>[2x]MDLTVEPNLHSLITSTTHKWIFVGGKGGVGKTTSSCSIAIQMALSQPNKQFLLIS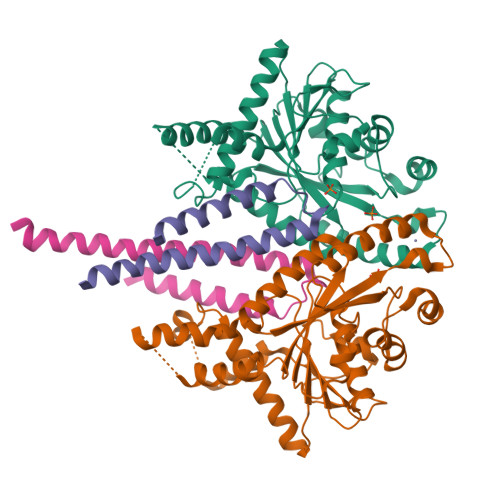TDPAHNLSDAFGEKFGKDARKVTGMNNLSCMEIDPSAALKDMNDMAVSRANNNGSDGQGDDLGSLLQGGALADLTGSIPGIDEALSFMEVMKHIKRQEQGEGETFDTVIFDTAPTGHTLRFLQLPNTLSKLLEKFGEITNKLGPMLNSFMGAGNVDISGKLNELKANVETIRQQFTDPDLTTFVCVCISEFLSLYETERLIQELISYDMDVNSIIVNQLLFAENDQEHNCKRCQARWKMQKKYLDQIDELYEDFHVVKMPLCAGEIRGLNNLTKFSQFLNKEYNPITDGKVIYELEDKELEHHHHHH;>[2x]MQYTNKYHEKWISKFAPGNELSKKYLAKVKERHELKEFNNSISAQDNYAKWTKNNRKLDSLDKEINNLKDEIQSENKAFQAHLHKLEHHHHHH The poly(ADP-ribose) polymerases (PARPs) Tankyrase (TNKS and ARTD5) and Tankyrase 2 (TNKS2 and ARTD6) regulate Wnt-β-catenin signaling (Huang et al., 2009). The two Tankyrases are highly similar (Hsiao and Smith, 2008, Smith et al., 1998), sharing a set of five ankyrin repeat clusters (ARCs) for substrate binding (Guettler et al., 2011, Seimiya et al., 2004), a sterile alpha motif (SAM) domain (De Rycker and Price, 2004, De Rycker et al., 2003), and a catalytic PARP domain (Rippmann et al., 2002). Tankyrase polymerization is mediated by the SAM domain, a small helical fold highly prevalent in eukaryotes (Knight et al., 2011, Qiao and Bowie, 2005). We report crystal structures of the polymerizing TNKS and TNKS2 sterile alpha motif (SAM) domains, revealing versatile head-to-tail interactions.

We also crystallized the TNKS SAM domain, which again required a polymer-breaking mutation. TNKS SAM D1055RT1, equivalent to D902RT2, produced two crystal forms in space group P21, diffracting to 2.5 Å (crystal form 1) and 2.9 Å (crystal form 2), both with six molecules in distinct asymmetric units. The TNKS SAM domain was highly similar to that of TNKS2 (left). For both TNKS crystal forms, non-crystallographic and crystallographic symmetry gave rise to left-handed helical filaments established by EH-ML contacts. The repeating unit consisted of six SAM domains with pitches of 83 and 79 Å, almost twice as long as for TNKS2. Unlike for TNKS2, where protomer contacts relied on crystallographic symmetry only and were therefore uniform, the TNKS SAM EH-ML contacts varied substantially. This was apparent from the merely approximate 6-fold axial symmetry and the variable tilt and twist between adjacent SAM domains. We conjecture that the variable relative orientations of SAM domains reflect filament flexibility. However, the equivalent residues (D1059T1, K1066T1, and K1081T1, respectively) mediated binding between a subset of protomers in the TNKS SAM crystal structures. Thus, contacts not seen in all SAM-SAM pairs are still generally relevant, probably occurring in some, but not all, configurations of the flexible filament.

>[6x]SNAERKEGEVAGLDMNISQFLKSLGLEHLRDIFETEQITLRVLADMGHEELKEIGINAYGHRHKLIKGVERLLGGQQGT N-{6-[3-(piperazin-1-yl)phenyl]pyridin-2-yl}-4-(trifluoromethyl)pyridin-2-amine | C21 H20 F3 N5 | 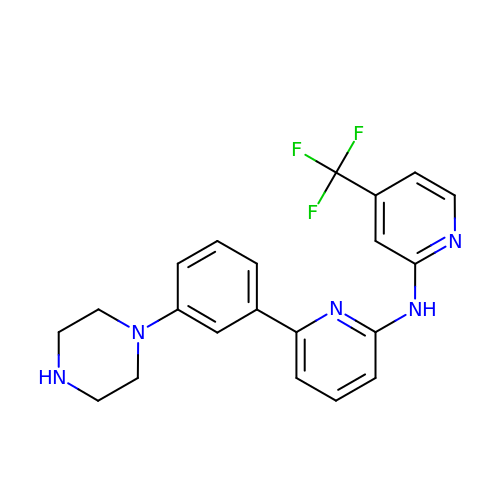FCPDILGNMHIWJE-UHFFFAOYSA-N N-[(2S)-2-amino-3-phenylpropyl]-D-methionyl-L-alanyl-L-isoleucine 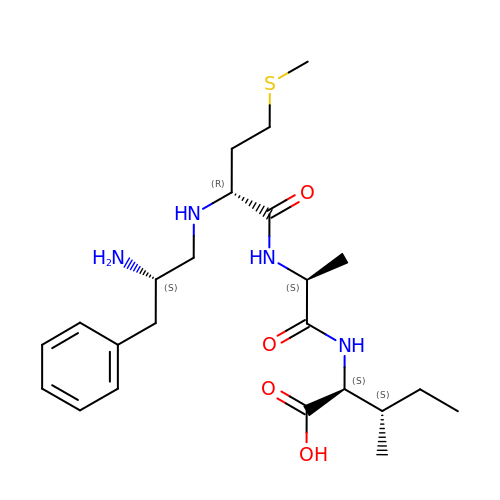| C23 H38 N4 O4 S | WTDYTUSSFIIXMV-HNULKUCHSA-N(4S)-1-(4-{[(2Z,4R)-4-(2-cyclohexylethyl)-4-(cyclohexylmethyl)-2-imino-5-oxoimidazolidin-1-yl]methyl}benzyl)-4-propylimidazolidin-2-one 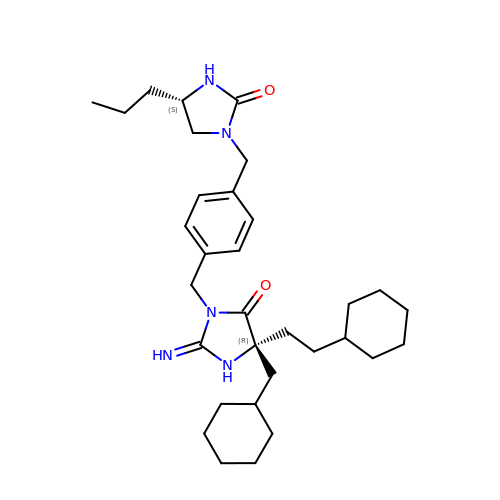| C32 H49 N5 O2 | SILGEXOUELDSRZ-GMCHKSTQSA-N> MAISKTNGQSKPKRKTEVPGQALGYSLQFTLLTHLLLQAPEGSLCSLEVLDDVAQENNSGDIKFIQSASALTANPAADRAKSLWKTLSNWIDLATSPDFEVEKAIFELYVSRPVEGSIVKKFNEAKTPEDAQEAITHARTELWGDSPHFTLKDGISKEISKYVEKVFTADQNLLQRLICNFQLTLGSGSPQADLEACVRSHPVSPSKVSDITNYLCGKVKRHIDMLLEAEKPAVIARDDFYTWYKAYVQKIDRQMVLSSRAQAPVKEKAQEYLPDKFVQQLEIIGLPYEEILGAISDYLMASFDRTDWAARGEVDETSFDDLDTALQRTWKNKQRICGLTHSEKSEQDQGKLLYFECMQFNIPLQAMSPPSHFIPGCYHILADSLAVGWHPNYTTQLKNKKVA;>MYFQIRGIILWPRNKNFKPHTIRFELGKVNVISGASRTGKSAVIPIIDYCLGANTCSIPVKTIRKYCEWFGIVVATEQGEKLLARKEPGNQRSTT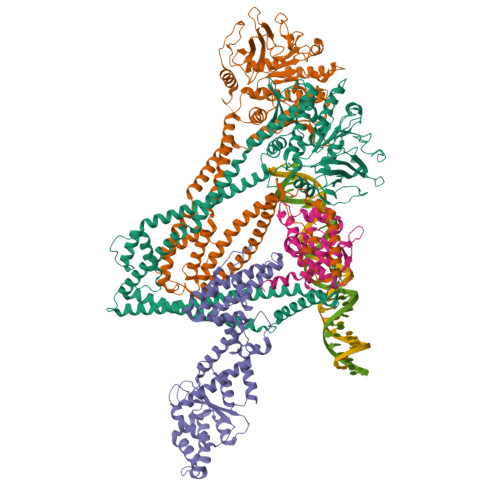DMFVLEAENITSIPIRLEKNTNVIAVKRMLDDLANLSNLDFSGGDENSGFDGRPAFRDLAAFTFQPQNVVANPDVLFFKTNTYEHREKLRKIFPYVLGAITSELMAKQFELNRIRLFLRRKERELKDAQDVSAQWLADLKSKYSEAQELGLVPKPQEQLSRKQMISQLEEVISRTDLTLKVTVSTISDALSELNTLESEERLVSRELTTMRHRLEEMNRLRVGMHQYENALLMQRDRLKISGWLLSNTNDESDCPMCGSHTDSAKQKLQALVQRLSDVEAAVGADAHKEVPAAFDRELQRVTTEVANATERLRAIQSRKRTLTSRSKEAREQQFSTRRAERFIGNVESALELHRKLGSDSELVEEVRKLKEMVQTLEKELREKDVELRKNQALRVINAQAGNILQGLDVEDPSAPISLEINDLTIKVLGDERDDYLSEIGSGSNWLSYHLAILLSLHQFYLSQKNNPVPSFLILDQPSQVYFPKTTQLPNIANEDEPKLRDEDVEAVRRAFKAMGNVVIKEKGKLQLIVLDHAPREVWGEIDGVVGLPEWRDGIKLVPMEWLTGV[2x];> MLAREAQNIQNPALGAALVWRFCCGYVKTNRVSAPPPLPFLFLVLPIILHQETSEFVKRTYKSSGLRAFAAKFGDSSVSKQDLLFQIHERSIRWRQLSLRSIELAVASDLLKLQDGSDVIPLSKTKARGLSDEVKTLMDLAEKLGSWFGELSIHEVVTTLKVKL>SNAMSNMQLDTLRRIVQEINSSVSLHDSLDIMVNQVADAM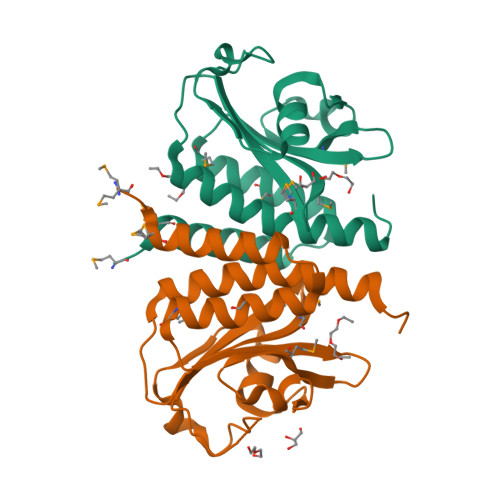KVDVCSIYLLDERNQRYLLMASKGLNPESVGHVSLQLSEGLVGLVGQREEIVNLENASKHERFAYLPETGEEIYNSFLGVPVMYRRKVMGVLVVQNKQPQDFSEAAESFLVTLCAQLSGVIAHAHAVGNID[2x]The methylation of lysine residues of histone proteins is a dynamic process that is regulated by SAM-dependent histone lysine methyltransferases, FAD- or Fe(II)/2OG-dependent histone demethylases, and reader proteins (also known as effector proteins) that specifically recognize post-translationally modified lysines in histones and affect the downstream cellular processes. The highest methylation state Kme3 is specifically recognized by a structurally diverse class of reader proteins, including plant homeodomain (PHD) zinc fingers, WD40 repeats and members of the Royal superfamily (tudor domain, chromodomain and PWWP domain), in the surface-groove binding mode. Our study reveals that the association between trimethyllysine and the aromatic cage of reader proteins is driven by energetically favourable cation–π interactions between the positively charged trimethyllysine and the electron-rich aromatic cage, and the trimethyllysine-mediated release of non-optimally structured water molecules that occupy the aromatic cages of reader proteins.

To elucidate the underlying chemical basis for the recognition of natural Kme3 by reader proteins, we have carried out detailed comparative studies for binding of 10-mer histone peptides that contain the positively charged Kme3, its neutral carba analogue Cme3, and the glycine residue that lacks the entire side chain at the fourth position of histone 3 (that is, H3K4me3, H3C4me3 and H3G4). We have chosen the simplest uncharged Cme3 analogue to directly probe the involvement of the proposed cation–π interactions in reader–histone associations, because it has virtually the same size, shape and polarizability as the positively charged Kme3, but lacks the presence of the fixed positive charge. We solved three X-ray crystal structures for complexes with JARID1A, TAF3 and SGF29 at 1.6–2.8 Å resolution. All three reader–H3C4me3 structures clearly illustrated that the uncharged side chain of C4me3 is positioned well inside the aromatic cages of JARID1A, TAF3 and SGF29, virtually in the same binding mode as the positively charged Kme3. The calculated average values of the root-mean-squared deviation for binding of ‘Cme3' and ‘Kme3'–aromatic cage pairs were: 0.124 Å for JARID1A, 0.261 Å for TAF3 and 0.108 Å for SGF29, respectively, suggesting essentially the same complexation mode engaging in aromatic pocket residues upon binding of neutral C4me3. Similar features have also been observed for binding of H3C4me3 and H3K4me3 to TAF3 with 48.3% buried SASA for H3C4me3 and 50.1% buried SASA for H3K4me3, and to SGF29 with 48.6 and 47.3% buried SASA for H3C4me3 and H3K4me3, respectively.

>[2x]GRRGVLMTLLQQSAMTLPLWIGKPGDKPPPLCGAIPASGDYVARPGDKVAARVKAVDGDEQWILAEVVSYSHATNKYEVDDIDEEGKERHTLSRRRVIPLPQWKANPETDPEALFQKEQLVLALYPQTTCFYRALIHAPPQRPQDDYSVLFEDTSYADGYSPPLNVAQRYVVACKEPKKK;>ARTXQTARKS[2x]> KLKEKENNDSSDKATVIPNFNTTMQGSLLGDDSR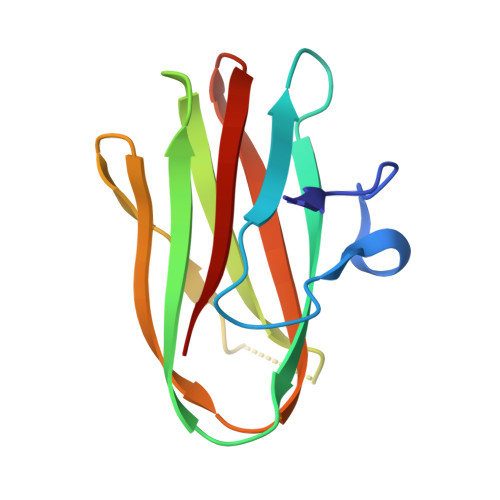DYYSFEVKEEGEVNIELDKKDEFGVTWTLHPESNINDRITYGQVDGNKVSNKVKLRPGKYYLLVYKYSGSGNYELRVNK Then, DBT sulfone monooxygenase DszA catalyzes the oxidation of DBT sulfone into 2′-hydroxybiphenyl 2-sulfonic acid (HBPSi). BdsA is a DBT sulfone monooxygenase that shares a 79% sequence identity with DszA from Rhodococcus sp. IGTS8. The BdsA monomer contains nine β-strands (β1–β9) and 13 α-helices (α1–α13), which fold into a triosephosphate isomerase (TIM)-barrel with five extended insertion regions. The TIM-barrel structure confirms that BdsA belongs to the group C flavin-dependent monooxygenases.

The structure of the tetrameric BdsA–FMN complex contains four FMN molecules, with each subunit binding one FMN. The binding pocket is mainly formed by IS1, IS2, IS3, and IS5. The overall Cα RMSD between apo-BdsA and the BdsA-FMN complex is only 0.240 Å. The most substantial structural discriminations were observed at the side chains of residues Phe56, Val137, and Phe246, which may facilitate the binding of FMN. The binding of FMN to BdsA is maintained through hydrogen bonds and hydrophobic interactions. The flavin ring of FMN lies in the barrel, with its plane nearly parallel with the staves of the barrel, and its si-face exposed to the solvent. There are several hydrogen bonding interactions between BdsA and FMN: the NE2 atom of His 156 with the O3 atom of the flavin phosphate groups (2.7 Å); the OG atom of Ser139 with the N1 atom of the flavin ring (2.8 Å); backbone nitrogen of Leu230 with the phosphate group (3.1 Å); and the Arg159 with the O4 atom of the flavin ring (3.4 Å). Two residues, Tyr160 and Val137, form van der Waals contacts with FMN. Based on the structural analysis, six single-point mutations of BdsA were constructed: V137A, S139A, H156A, R159A, Y160A, and L230A. The results of enzymatic activity showed that mutant proteins V137A, S139A, R159A, Y160A, and L230A completely lost their activity.

>MAEQRQLHLAGFFSAGNVTHAHGAWRHVGATNGFLTGEFYKQIARTLERGKFDLLFLPDGLAIEDSYGDNLETGVGLGGQGAVALEPTSVIATMAAVTQRLGLGATVSTTYYPPYHVARVFATLDNLSDGRISWNVVTSLNDSEARNFGVDEHLEHDIRYDRADEFLEAVKKLWSSWSEDALLLDKVGGRFADPKKVQYVNHRGRWLSVRGPLQVPRSRQGEPVILQAGLSPRGRRFAGRWAEAVFSVSPNLDIMRAVYQDIKAHVAAAGRDPEQTKVFTAVMPVLGETEQVARERLEYLNSLVHPEVGLSTLSSHSGLNLSKYPLDTKFSDIVADLGDRHVPTMLQMFSAVAGGGADLTLAELGRRYGTNVGFVPQWAGTAEQIADQLISHFEAGAADGFIISPAYLPGIYEEFVDQVVPLLQQRGVFRTEYEGTTLREHLGLAHPEVGSIR[4x]>[2x]MTTATAGLAVELKQSTAQAHEKAEHSTFMSDLLKGRLGVAEFTRLQEQAWLFYTALEQAVDAVRASGFAESLLDPALNRAEVLARDLDKLNGSSEWRSRITASPAVIDYVNRL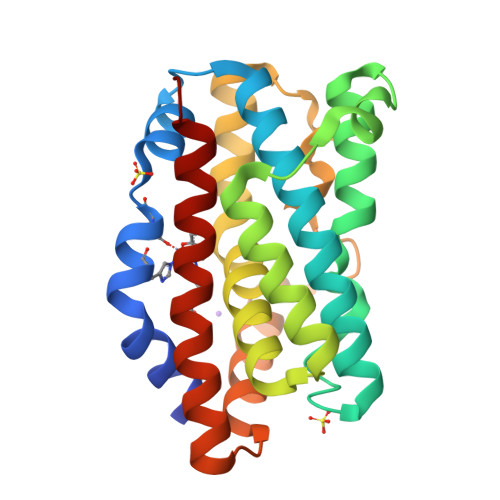EEIRDNVDGPALVAHHYVRYLGDLSGGQVIARMMQRHYGVDPEALGFYHFEGIAKLKVYKDEYREKLNNLELSDEQREHLLKEATDAFVFNHQVFADLGKGL3,5-dichlorobenzene-1,2-diol | C6 H4 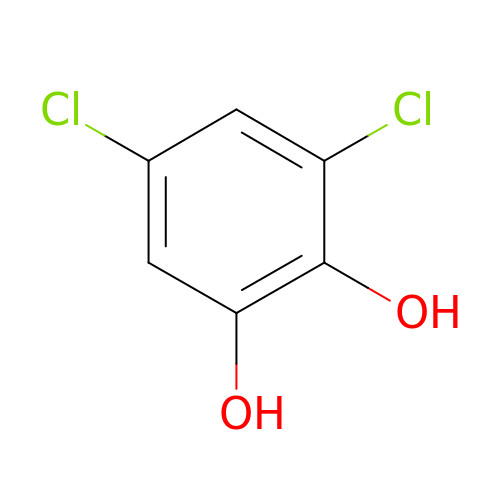Cl2 O2 | XSXYVLIPQMXCBV-UHFFFAOYSA-N>[2x]GETKEDIARKEQLKSLLPPLDNIINLYDFEYLASQTLTKQAWAYYSSGANDEVTHRENHNAYHRIFFKPKILVDVRKVDISTDMLGSHVDVPFYVSATALCKLGNPLEGEKDVARGCGQGVTKVPQMISTLASCSPEEIIEAAPSDKQIQWYQLYVNSDRKITDDLVKNVEKLGVKALFVTVDAPSLGQREKDMKLKFSN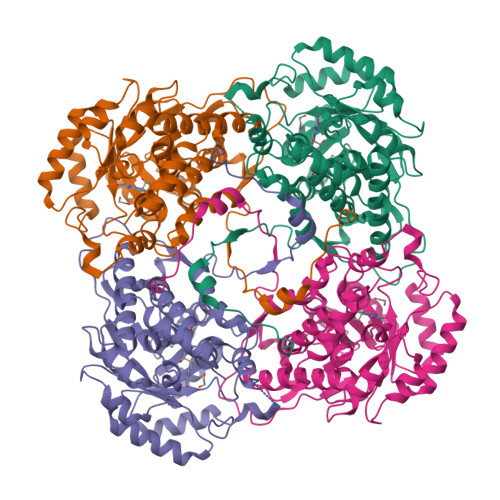TKAGPKAMKKTNVEESQGASRALSKFIDPSLTWKDIEELKKKTKLPIVIKGVQRTEDVIKAAEIGVSGVVLSNHGGRQLDFSRAPIEVLAETMPILEQRNLKDKLEVFVDGGVRRGTDVLKALCLGAKGVGLGRPFLYANSCYGRNGVEKAIEILRDEIEMSMRLLGVTSIAELKPDLLDLSTLKARTVGVPNDVLYNEVYEGPTLTEFEDA> GSAAQYGRALQAMEANKYDEARKTLQPLLAAEPGNAWYLDLATDIDLGQNKANEAINRLKNARDLRTNPVLQLNLANAYLQGGQPQEAANILNR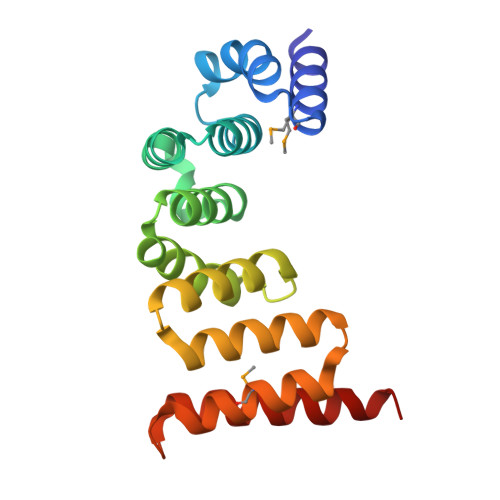YTFNNKDDSNGWDLLAQAEAALNNRDQELAARAEGYALAGRLDQAISLMSSASSQVKLGSLQQARYDARIDQLRQLQERFK>MDKAETSSMAEAESEDSETTTPTTHHLTIPPGLTQPEFQELAHSISEFHTYQVGPGQCSSLLAQRVHAPLPTVWSVVRRFDKPQTYKHFIKSCHVEDGFEMRVGCLRDVNVISGLPAETSTERLDILDDERHVTGFSIIGGEHRLRNYRSVTTVHEYQNHGGEIWTVVLESYVVDMPEGNTEEDTRLFADTVVKLNLQKLASVTEGMAR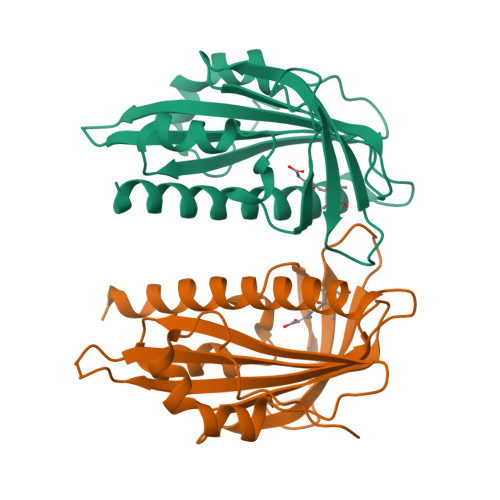DQGCF[2x]> AHMNTHSGGETQVWEVWMYSQSEKKHRSKSLKMYNSLIIADPGPSLAVSDRCVAIVL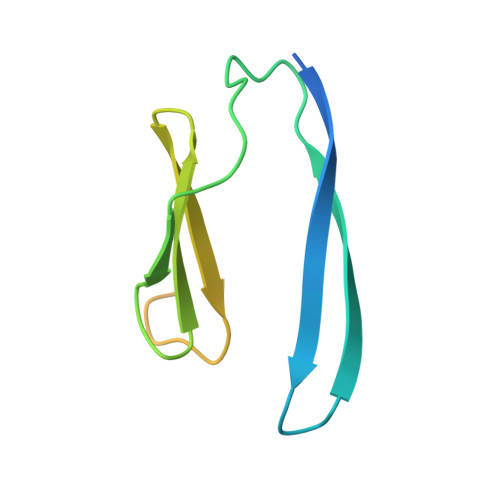GNYVALVGYGSEIFRDFYQIRNSDEMDRILRRKRKNLQRKRSGTIG> SGSGSWQTYVDD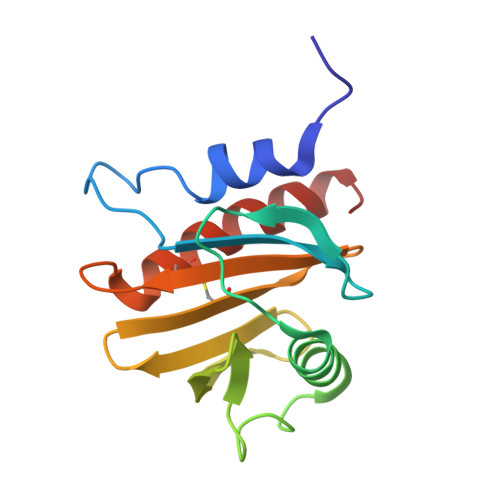HLMCDIEGTGQHLTSAAIFGTDGTVWAKSASFPEFKPNEIDAIIKEFNEAGQLAPTGLFLGGAKYMVIQGEAGAVIRGKKGAGGICIKKTGQAMVFGIYDEPVAPGQCNMVVERLGDYLLDQGM>MSLSKSLQKPTILNVETVARSRLFTVESVDLEFSNGVRRVYERMRPTNREAVMIVPIVDDHLILIREYAVGTESYELGFSKGLIDPGESVYEAANRELKEEVGFGANDLTFLKKLSMAPSYFSSKMNIVVAQDLYPESLEGDEPEPLPQVRWPLAHMMDLLEDPDFNEARNVSALFLVREWLKGQGRVEGGSHHHHHH[2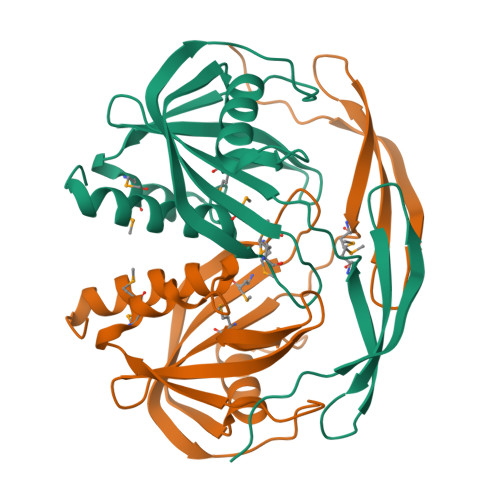x]>[2x]LPQASIDLTPQTFNEKVLQGKTHWV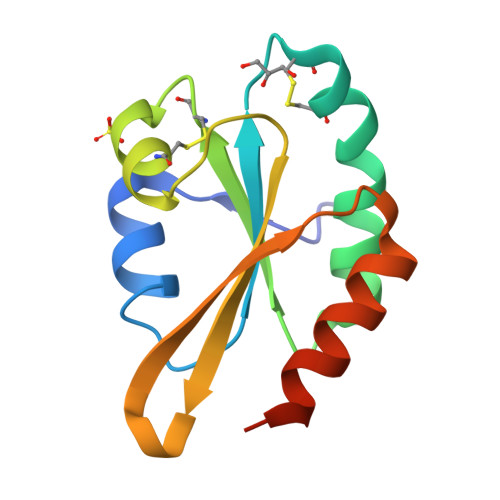VDFYAPWCGPCQNFAPEFELLARMIKGKVRAGKVDCQAYPQTCQKAGIKAYPSVKLYQYERAKKSIWEEQINSRDAKTIAALIYGKLETLQSQVKRN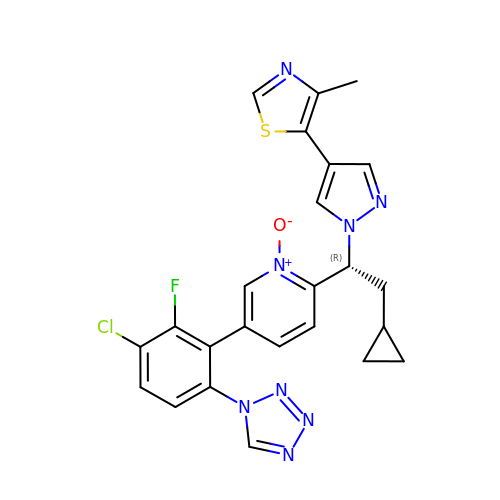5-[1-[(1~{R})-1-[5-[3-chloranyl-2-fluoranyl-6-(1,2,3,4-tetrazol-1-yl)phenyl]-1-oxidanyl-pyridin-2-yl]-2-cyclopropyl-ethyl]pyrazol-4-yl]-4-methyl-1,3-thiazole | C24 H20 Cl F N8 O S | LVFYRSDTZFJORD-OAQYLSRUSA-N>[2x]ANSMSVEAAKNARELLLKEYRAVLSTHSKKWPGFPFGSVVPYCLDAEGRPLILISRIAQHTHNLQADPRCSMLVGERGAEDIQAVGRLTLLAEARQLAEEE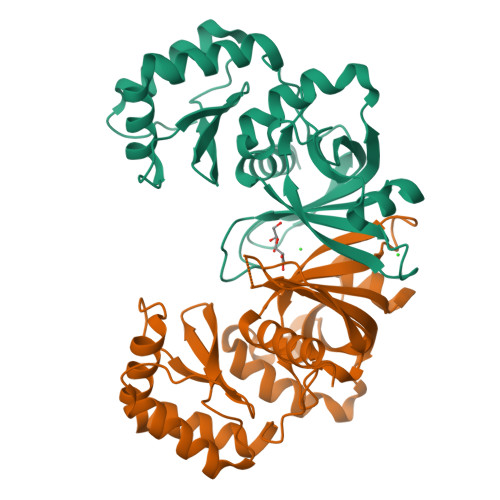VAAAAERYYRYFPESADYHRVHDFDFWVLQPVQWRFIGGFGAIHWLAAERVPLANPFAGEAERGMVEHMNSDHAAAIAHYVELAGLPAHAAAQLAGIDTEGFHLRIGQGLHWLPFPAACGNPGAVRQALVQLARAERWPTVEPEQG> MVVKAAGLVIYRKLAGKIEFLLLQASYPPHHWTPPKGHVDPGEDEWQAAIRETKEEANITKEQLTIHEDCHETLFYEAKGKPKSVKYWLAKLNNPDDVQLSHEHQNW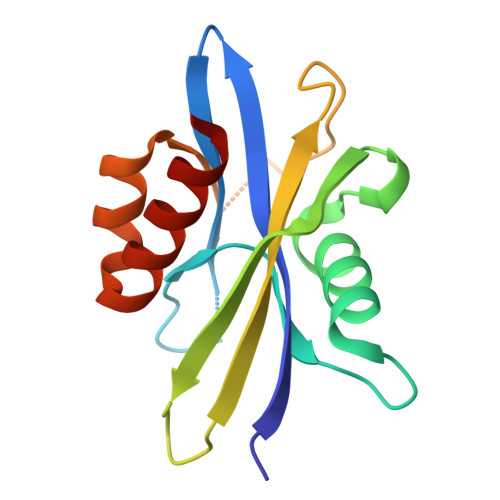KWCELEDAIKIADYAEMGSLLRKFSAFLAGF>TKPLDGINVLDFTHVQAGPACTQMMGFLGANVIKIERRGSGDMTRGWLQDKPNVDSLYFTMFNCNKRSIELDMKTPEGKELLEQMIKKADVMVENFGPGALDRMGFTWEYIQELNPRVILASVKGYAEGHANEHLKVYENVAQCSGGAAATTGFWDGPPTVSGAALGASNSGMHLMIGILAALEIRHKTGRGQKVAVAMQDAVLNLVRIKLRDQQRLERTGILAEYPQAQPNFAFDRDGNPLSFDNITSVPRGGNAGGGGQPGWMLKCKGWETDADSYVYFTIAANMWPQICDMIDKPEWKDDPAYNTFEGRVDKLMDIFSFIETKFADKDKFEVT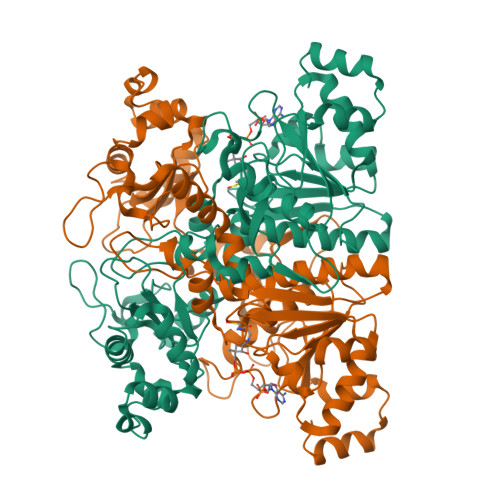EWAAQYGIPCGPVMSMKELAHDPSLQKVGTVVEVVDEIRGNHLTVGAPFKFSGFQPEITRAPLLGEHTDEVLKELGLDDAKIKELHAKQVV[2x]> MKPESKEAPINIRAKASQRDLIDMAANLVAKSRTDFM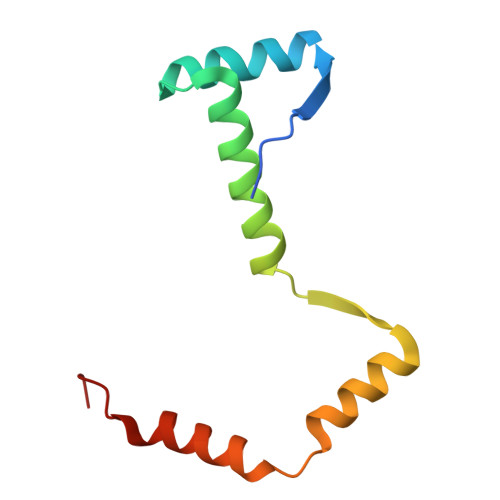LDAACREAQDILLDQRLFILDDEQYDAFLAALDAPITAERQAKINALMNRKSPWE>[3x]MNMPNERLKWLMLFAAVALIACGSQTLAANPPDADQKGPVFLKEPTNRIDFSNSTGAEIECKASGNPMPEIIWIRSDGTAVGDVPGLRQISSDGKLVFPPFRAEDYRQEVHAQVYACLARNQFGSIISRDVHVRAVVAQYYEADVNKEHVIRGNSAVIKCLIPSFVADFVEVVSWHTDEEENYFPGAEYDGKYLVLPSGELHIREVGPEDGYKSYQCRTKHRLTGETRLSATKGRLV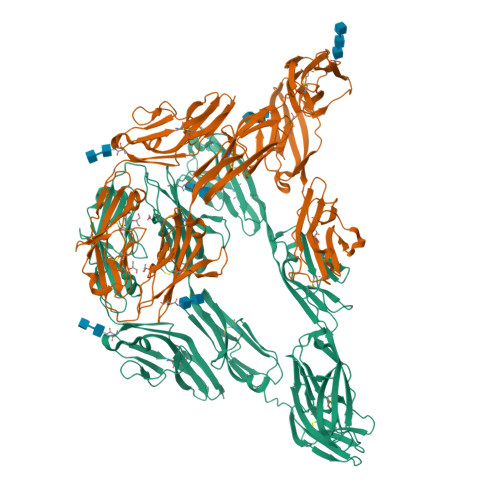ITEPISSAVPKVVSLAKFDMKTYSGSSTMALLCPAQGYPVPVFRWYKFIEGTTRKQAVVLNDRVKQVSGTLIIKDAVVEDSGKYLCVVNNSVGGESVETVLTVTAPLSAKIDPPTQTVDFGRPAVFTCQYTGNPIKTVSWMKDGKAIGHSESVLRIESVKKEDKGMYQCFVRNDRESAEASAELKLGGRFDPPVIRQAFQEETMEPGPSVFLKCVAGGNPTPEISWELDGKKIANNDRYQVGQYVTVNGDVVSYLNITSVHANDGGLYKCIAKSKVGVAEHSAKLNVYGLPYIRQMEKKAIVAGETLIVTCPVAGYPIDSIVWERDNRALPINRKQKVFPNGTLIIENVERNSDQATYTCVAKNQEGYSARGSLEVQVMVLPRIIPFAFEEGPAQVGQYLTLHCSVPGGDLPLNIDWTLDGQAISEDLGITTSRVGRRGSVLTIEAVEASHAGNFTCHARNLAGHQQFTTPLNVYVPPRWILEPTDKAFAQGSDAKVECKADGFPKPQVTWKKAVGDTPGEYKDLKKSDNIRVEEGTLHVDNIQKTNEGYYLCEAINGIGSGLSAVIMISVQAHHHHHH> SNAMSSMQFTDKATETLNAAAKYAAENSHVQLHPSHVAVVMLDEENSLFRSILEKAGGDVVSIERGFKKIMVRQPSQDPPPTEMGHSPELAKLLHYAHEHMKKQRDLYIAQDHLILALADLPSMAQVLKEGGVTKKSLENAVTHVRGNRRVESKSAEEAYEALSKYCIDLTELAASGKLDPVIGRDEIISRVIRVLSRRTKNNPCLVGEPGVGKTAIAEGLANRIVKGDIPSSLQKKVYSLDIGSLLAG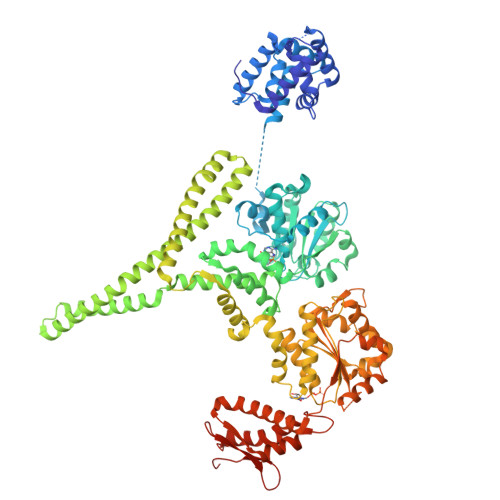AKYRGEFEERLKAVLKELKEAQAIVFIDEIHTVLGAGKSEGAIDAANLLKPMLARGELRCIGATTLTEYRQYVEKDPAFERMFQLVMVEEPSVTDTISILRGLKERYETHHGVRIADAAIVAAAQLAARYITQRFMPDKAIDLIDEACANTRVQLDSQPEAIDKLERRHLQLEVEATALEKEKDAASKQRLQEVRAEMARIQEELRPLKMKYESEKGRLDEIRNLSQRLDELKAKAEDAERRYDLARAADIRYYAIPDLEKRLAQLQAEKSQADAERADGLLAEVVGPDQIMEVVSRWTGIPVSNLQRSEKEKLLHMEEYMKQHVVGQDEAIKAICDAIRLSRTGLQNRNRPLASFLFLGPTGCGKTLCVKELAAFLFNDPGAIVRIDMSEYMEKHAVSRLVGAPPGYIGHDEGGQLTEAVRRRPYTVVLFDEMEKAHKDVSNLLLQILDDGHCTDSKGRRVDFKNTIIVMTSNLGADLFELDEGDKVSQATKNAVLATARRHFANEFINMIDELIVFNRLTPSNIRKIVDVRLKEVQERLDEKQITLDVDDKAKDLLAQQGFDPVYGARPLNRLIQHALLTQLSRLLLDGGVRPGEIAKVTVDQEGEIIVIRNHGIESPAPWADEDMVEDEDMEI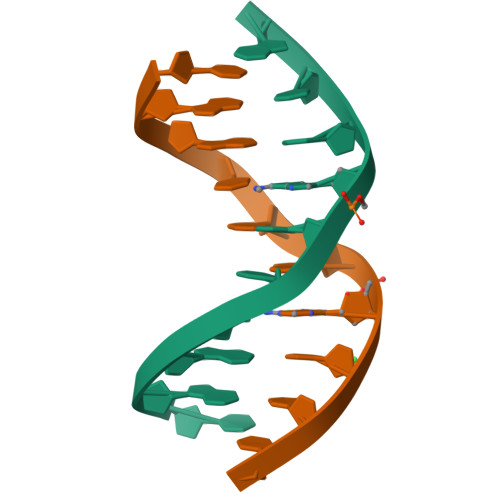>CGATCGATCG[2x]> SYDPCTERYSTAYYNRRDVQMALHANVTGAMNYTWATCSDTINTHWHDAPRSMLPIYRELIAAGLRIWV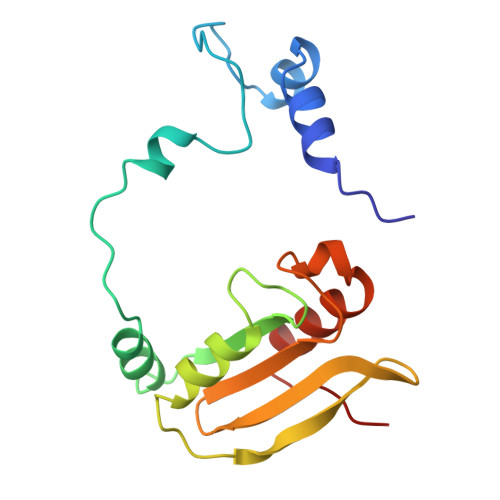FSGDTDAVVPLTATRYSIGALGLPTTTSWYPWYDDQEVGGWSQVYKGLTLVSVRGAGHEVPLHRPRQALVLFQYFLQGKPMPGQ> GPVWRKHYITYRINNYTPDMNREDVDYAIRKAFQVWSNVTPLKFSKINTGMADILVVFARGA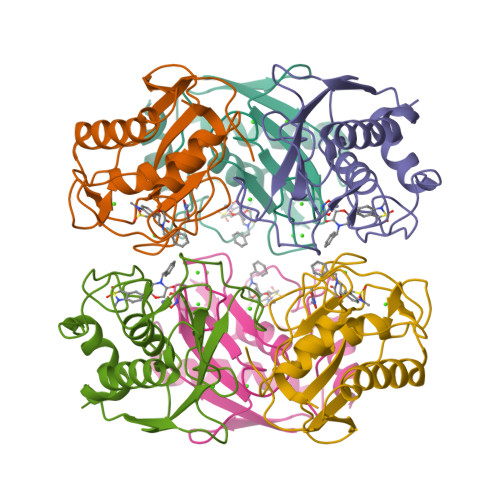HGDFHAFDGKGGILAHAFGPGSGIGGDAHFDEDEFWTTHSGGTNLFLTAVHEIGHSLGLGHSSDPKAVMFPTYKYVDINTFRLSADDIRGIQSLYGD>MKNKVVVVTGVPGVGGTTLTQKTIEKLKEEGIEYKMVNFGTVMFEVAKEEGLVEDRDQMRKLDPDTQKRIQKLAGRKIAEMAKESNVIVDTHSTVKTPKGYLAGLPIWVLEELNPDIIVIVETSSDEILMRR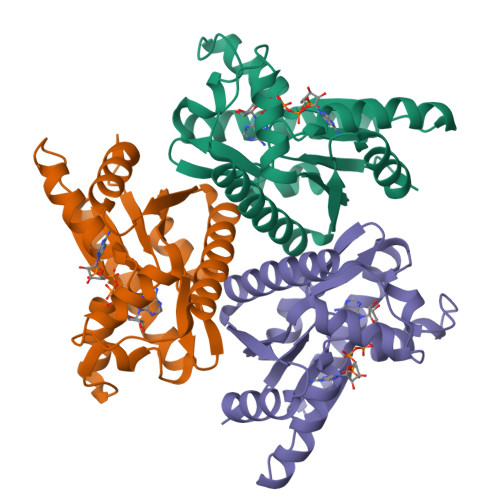LGDATRNRDIELTSDIDEHQFMNRCAAMAYGVLTGATVKIIKNRDGLLDKAVEELISVLKLEHHHHHH[6x]The Sumo-specific E1 enzyme [the heterodimeric complex between Uba2 and Aos1 (yeast; termed Sae1-Uba2 in mammals)] initiates the process by first catalyzing adenylation of the Sumo C-terminus, which next becomes linked by a thioester bond to Uba2's catalytic cysteine. A transthiolation reaction ensues during which Sumo is transferred from Uba2 to the catalytic cysteine of the dedicated Sumo E2 conjugating enzyme, Ubc9. In addition, for both yeast and human Uba2, the ufd has been implicated in Ubc9 recruitment. Therefore, to obtain a more detailed understanding of Uba2's ufd interactions with Ubc9 and to obtain broad insights into how E1-E2 specificity is established in general, we performed structural analysis of the Uba2ufd-Ubc9 complex from S. cerevisiae.

Like ubiquitin and Sumo, the Uba2ufd adopts a modified β-grasp fold. Uba2ufd consists of a twisted 5-stranded antiparallel β-sheet on one side, one 3-turn α-helix on the opposite side of the sheet, and two peripheral short helices. The β-sheet and connecting loops form one V-shaped surface. The two V-like structures are adjacent to each other, and together form a W-shaped surface. The structure of the Uba2ufd is nearly identical in the complex as on its own (0.47 Å rmsd). The Uba2ufd C-terminal “V” is minimized relative to the corresponding regions in ubiquitin and NEDD8 E1s, which would be unable to accommodate the Ubc9 β1β2-loop.

> GSSKVCRGVIKLSSDCLNKMKLSDFVVLIREKYSYPQDISLLDASNQRLLFDYDFEDLNDRTLSEINLGNGSIILFSDEEGDTMIRKAIELFLDVDDELPCNTCSLPDVEVPLIKANNSPSKNEEEE> ADLGSPCGGRLNSKDAGYITSPGYPQDYPSHQNCEWIVYAPEPNQKI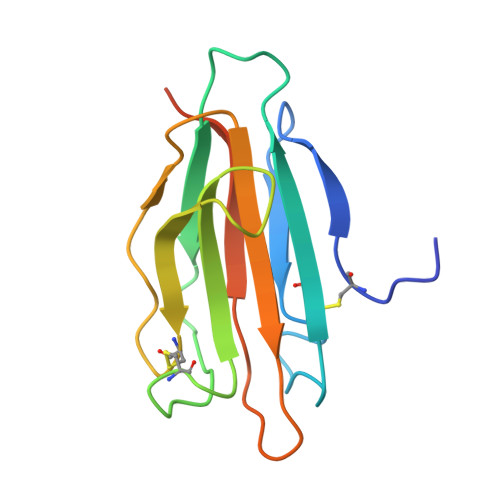VLNFNPHFEIEKHDCKYDFIEIRDGDSESADLLGKHCGNIAPPTIISSGSMLYIRFTSDYARQGAGFSLRYEIFKTGSGTHHHHHH> GICPRFAHVIENLLLGTPSSYETSLKEFEPDDTMKDAGM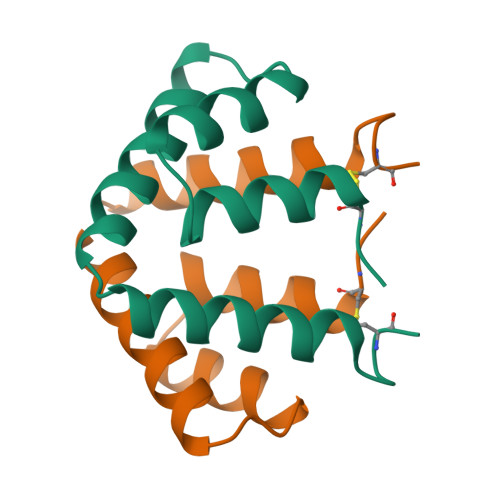QMKKVLDSLPQTTRENIMKLTEKIVKSPLCM The H3/H4 chaperone CAF-1 is conserved among all eukaryotes and has important roles during DNA replication and repair, regulation of gene expression, and maintenance of chromatin accessibility. The budding yeast CAF-1 complex consists of subunits Cac1, Cac2, and Cac3, which differ in their ability to bind H3/H4. The data indicate that Cac1 is the major subunit required and is sufficient for binding and tetramerizing H3/H4. Rather, the Cac1 glutamate/aspartate (ED) domain is also required to tetramerize H3/H4 in vitro. These results support an architectural model for the replication-coupled CAF-1-H3/H4 complex, in which Cac1 scaffolds all protein-protein interactions and is predominantly involved in H3/H4 tetramerization.

Although this putative dimerization sequence is apparently not conserved in yeast, purified S. cerevisiae Cac1 elutes from size exclusion chromatography at a molecular weight consistent with a dimer, confirmed by multiangle light scattering. To gain structural insight into the putative Cac1 dimer, we crystallized E. coli-expressed Cac1457, a region that forms many stable intra-Cac1 chemical cross-links. The structure was determined using molecular replacement to a resolution of 2.9 Å with coordinates from a recently determined structure of Cac1C (522–600). Even though the entire 457–606 protein was present in the crystal (Figure 5A and data not shown), only amino acids 520–600 were visible in our electron density, and the 'wing' (576–581) was disordered. As expected, the structure we determined is virtually identical to the reported Cac1C winged helix (WH) domain, with an overall root mean squared deviation (r.m.s.d.) of 1.14 Å for all atoms. Indeed, we observed a crystallographic homo-dimer. The inset shows major interacting residues buried in half of the homodimer interface, which is arranged in a head-to-tail symmetry with identical interactions on both halves. The putative dimerization domain consists of residues 572–600 at the C-terminus, and does not appear to extend to amino acid 386, as Cac1386(Py) and Cac1454(Py) have similar dimerization constants. Therefore, Cac1 dimerization is not necessary to promote (H3/H4)2 tetramerization, consistent with the functional stoichiometry of CAF-1. Thus, the WH domain exhibits binding plasticity for different partners.

> SNFENLSEENKRYLQQLKAEVIIETDGPIDPFKEPKTSSLPSKRSNSDLQAQTASQSQSPEKKQKAMITDPMDLLRLFDGVQDSTFSLGTVTEIAQKNLPQYNKQTIKNTIKEYAIRSSGKGDLPRKWVIKDAQNWENLRANANMPTPSL> SSQPNATLYKMSSINADFAFNLYRRFTVETPDKNIFFSPVSISAALVMLSFGACCSTQTEIVETLGFNLTDTPMVEIQHGFQHLICSLNFPKKELELQIGNALFIGKHLKPLAKFLNDVKTLYETEVFSTDFSNISAAKQEINSHVEMQTKGKVVGLIQDLKPNTIMVLVNYIHFKAQWANPFDPSKTEDSSSFLIDKTTTVQVPMMHQMDQYYHLVDMELNCTVLQMDYSKNALALFVLPKEGQMESVEAAMSSKTLKKWNRLLQKGWVDLFVPKFSISATYDLGATLLKMGIQHAYSENADFSGLTEDNGLKLSNAAHKAVLHIGEKGTEAAGAMFLEAIPRSIPNTF;> LHPIIQI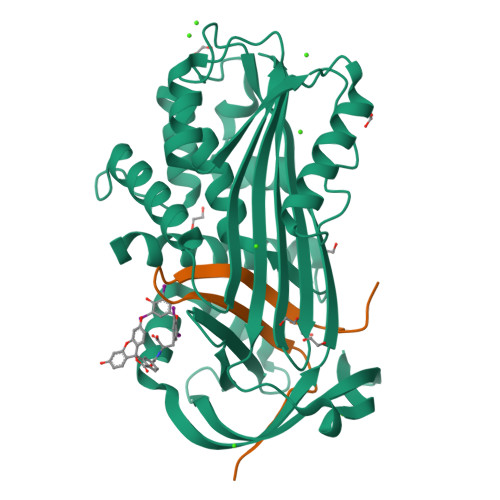DRSFMLLILERSTRSILFLGKVVNPTEA> MPSSRRVRSRCCAFGITKRFACI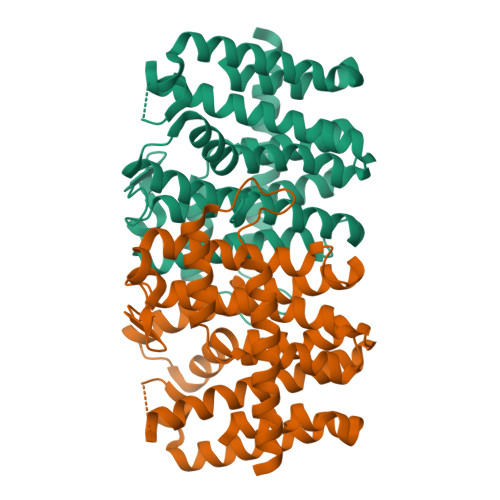RPACQRARMDAQMTNFETRLRENAAKTEALLGHLLSGEARADEITRPQNLLEAMRHGVLNGGKRLRPFLVIESVALLGGDAEAGLHVGAALECLHCYSLVHDDLPAMDDDDLRRGQPTVHRKFDEATAILAGDSLLTLAFDIIASDDNPLAAERKAALVISLARAAGIGGMAGGQALDLAAEKKAPDEDGIITLQAMKTGALLRFACEAGAIIAGSNQAERQRLRLFGEKIGLSFQLADDLLDLTADAATMGKATGKDAARGKGTLVALRGEAWAREKLQEQVAEASELLAPYGEKAAILIAAARFIAERKS>[2x]MTHRKQPSSSSKLPDSILKRGAEASKVLEEHLERGNIIRIISHNDADGLSAAGVVARAISSMNGQFHISILSRLKKEFIKKLSGEKYSLFFFCDMGSAYLEEISRLKGDVIVADHHQPS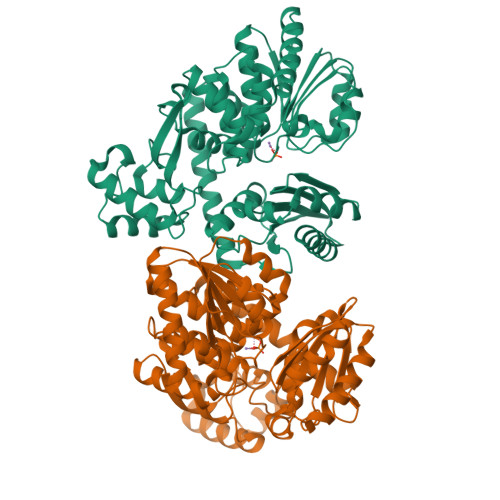ESEAGPHVVHINPHLHGLDGSRDLSASGTAYLATRLLNRKTAPLALVGALGDMQYTDGFTGANRFIMEEAVEEGVLQVHSDLKLASRYTEPLYRSIAYTFNPALPGLTGDMEASMGFLENIGVSYGVKYPDLSPEERDVLRDELTRINPEIFGEVFTSREFRNIGDLSDIAGVLDACGKNRKYGIGIGLCLGEREGALDVALELQKNYREELVKGLAWIRREGSTTLENLQYIYSEDKAFKGIMGTIASISLSLKILDPDIPLLGLSRMDQHVKVSARTTRPAVERGVNLGVALRDAAASFGGTGGGHDIAAGAMVPYRDMESFLQLVDEILGTQTGPAENLYFQ2-chloro-4-[(2S,3S)-3-hydroxy-2-methylpyrrolidin-1-yl]-3-methylbenzonitrile | C13 H15 Cl N2 O 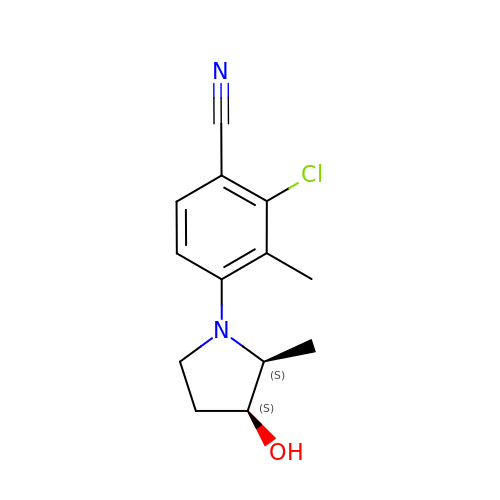| SSTNLJGXVPIZND-CABZTGNLSA-N>MSPILGYWKIKGLVQPTRLLLEYLEEKYEEHLYERDEGDKWRNKKFELGLEFPNLPYYIDGDVKLTQSMAIIRYIADKHNMLGGCPKERAEISMLEGAVLDIRYGVSRIAYSKDFETLKVDFLSKLPEMLKMFEDRLCHKTYLNGDHVTHPDFMLYDALDVVLYMDPMCLDAFPKLVCFKKRIEAIPQID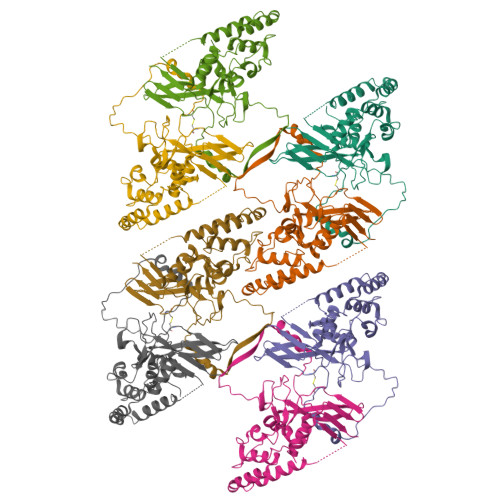KYLKSSKYIAWPLQGWQATFGGGDHPPKSDLEVLFQGPLGSGGGGGMALVTVPTATTRLRNFCVFSSVKPLDFCDQYSSPCSSDATVDDGWFVCEYHASRFFKMEKLALAIPDGTGNNYYRTVGKSLVDDKAEGIERILIPSQNNYETVLNLSLLGPAERLVFYMIYDNKEKQNEICQQLRMYERFRPEVVEELYNSTLRVLALTNPDAYCAQTNTNESRSFGLSVEDDLAFNVLPTFIQNLIRKCVAPESLTIGTEDLQLRNCNTCRITSEGLLASVRLYNSVQPKYLYGVNENRLQIRNVLQFQGNANALQQKLSRYELYQINIPLFLGKQIISTGC[8x]> PALRANIQQALNHITKNIHLTQAQMEDVMRSIMQGNATEAQIGALMMGLRMKGESIDEITAAARVMRELAIKIDVSDIQYLVDIVGTGGDGQNLFNVSTASSFVIAAAGATIAKHGNRGVSSKSGSSDLLEQAGINLDLDMQQTERCIREMGVGFLFAPNHHKAMKYAVGPRRELGIRSIFNLLGPLTNPAGVKRFVIGVFSDELCRPIAE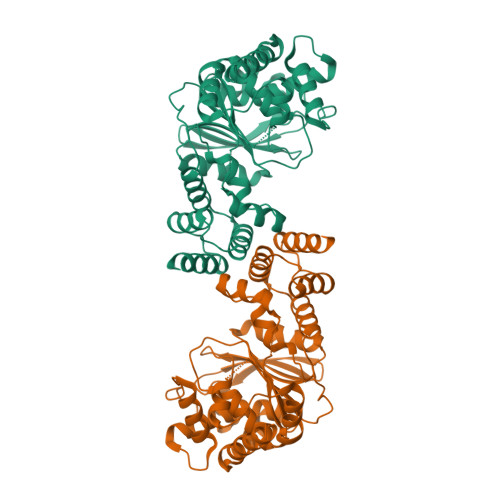VMKQLGAEHVMVVHSKDGLDEISLASQTYIAELKNGEVTEWVLNPEDVNIPSQTLSGLIVEDSNASLKLIKDALGRKKSDIGEKAANMIALNAGAGIYVSGLATSYKQGVALAHDIIYGGQALEKMSILSEFTKALKEYANN>[2x]SNAMSQQVTMSFSVVPQAKTKDVYSVVDKAIEVVQQSGVRYEVGAMETT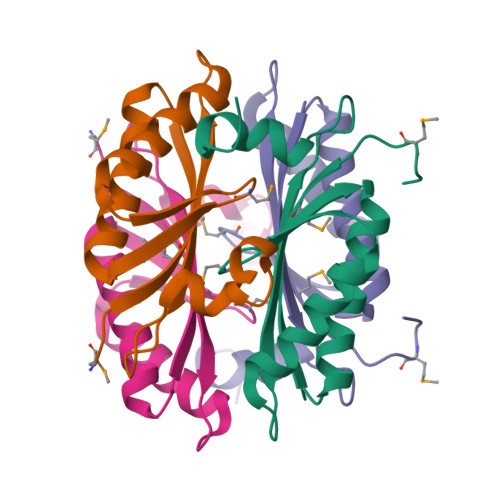LEGELDVLLDVVKRAQQACVDAGAEEVITSIKIHYRPSTGVTIDEKVWKYRDEYAKPEAI>APMKLYGAVMSWNLTRCATALEEAGSDYEIVPINFATAEHKSPEHLVRNPFGQVPALQDGDLYLFESRAICKYAARKNKPELLREGNLEEAAMVDVWIEVEANQYTAALNPILFQVLISPMLGGTTDQKVVDENLEKLKKVLEVYEARLTKCKYLAGDFLSLADLNHVSVTLCLFAT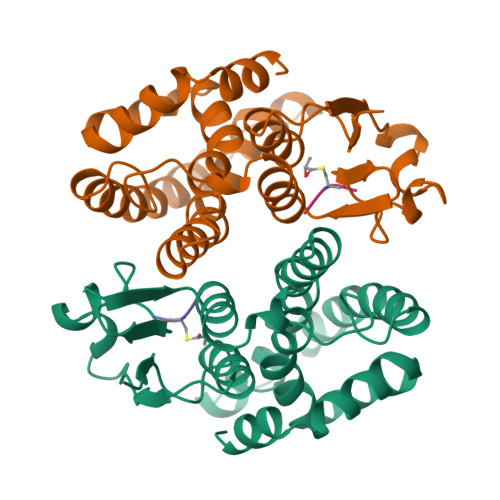PYASVLDAYPHVKAWWSGLMERPSVQKVAALM[2x]> MGQNTLKVHDLNEDAEFDENGVEVFDEKALVEE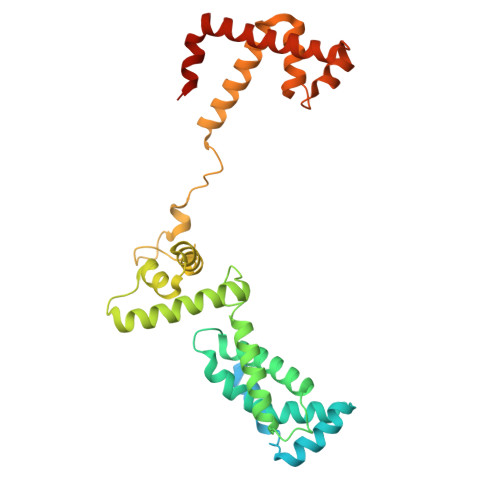EPSDNDLAEEELLSQGATQRVLDATQLYLGEIGYSPLLTAEEEVYFARRALRGDVASRRRMIESNLRLVVKIARRYGNRGLALLDLIEEGNLGLIRAVEKFDPERGFRFSTYATWWIRQTIERAIMNQTRTIRLPIHIVKELNVYLRTARELSHKLDHEPSAEEIAEQLDKPVDDVSRMLRLNERITSVDTPLGGDSEKALLDILADEKENGPEDTTQDDDMKQSIVKWLFELNAKQREVLARRFGLLGYEAATLEDVGREIGLTRERVRQIQVEGLRRLREILQTQGLNIEALFLEHHHHHH>MDHHHHHHENLYFQMEPEESMMGMKETVSNIVTSQAEKGGVKHVYYVACGGSYAAFYPAKAFLEKEAKALTVGLYNSGEFINNPPVALGENAVVVVASHKGNTPETIKAAEIARQHGAPVIGLTWIMDSPLVAHCDYVETYTFGDGKDIAGEKTMKGLLSAVELLQQTEGYAHYDDFQDGVSKINRIVWRACEQVAERAQAFAQEYKDDKVIYTVASGAGYGAAYLQSICIFMEMQWIHSACIHSGEFFHGPFEITDANTPFFFQFSEGNTRAVDER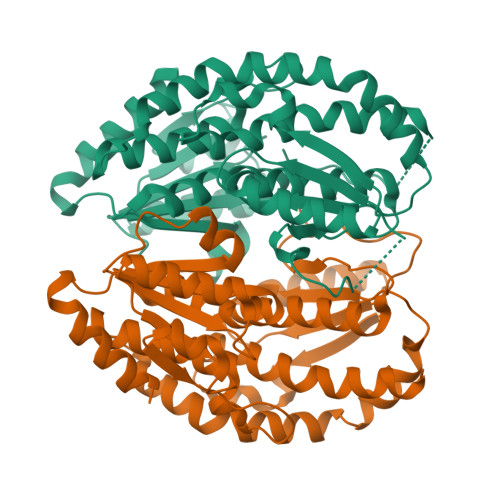ALNFLKKYGRRIEVVDAAALGLSTIKTTVIDYFNHSLFNNVYPVYNRALAEARQHPLTTRRYMWKVEY[2x]> MDNKIAGYNIIIHTIISSINMKFSLVVLSSLVVASSNGVTAFAPSSSTTSTSTTALSSSASKAELEAIAKKANPTLGYYDPLSLADKDFWGKGNDATIAFLRQSEIKHGRIAMFAFVGYIVQSNFVFPWAQTLAGAPHPSADLSPEAQWDAIPLGAKWQIFAVISALELWD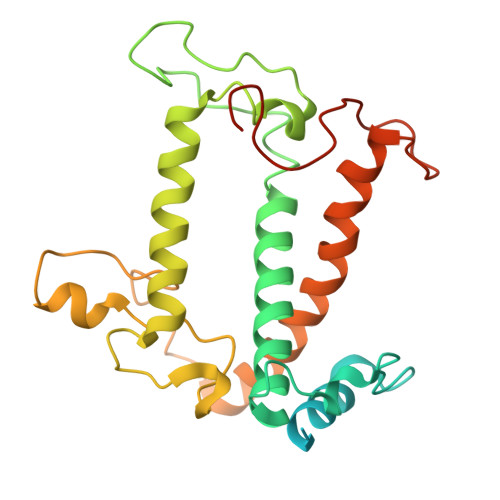ECGGGGVLPHYTKGRKPGQYPPFTLFRDNVHFVLDLYDPFGFNKNMSEETKERRLVSELNNGRLAMLGIFGFLCADTIPGSVPLLNDIAIPYSGQVMQPFEGQFSYFGSL>DSYVHRHVVTFDETNLVGNV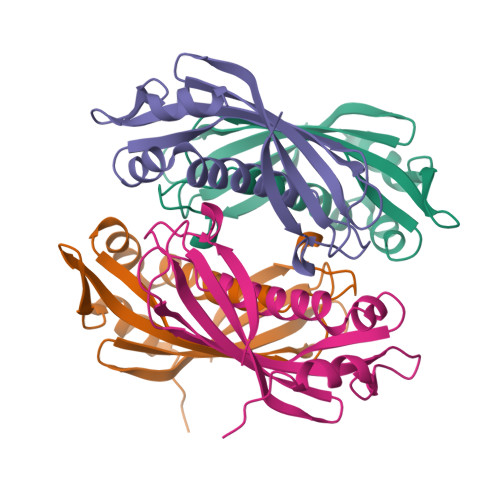YFAHYLHWQGHCREHFLADHAPGVMAALADGLALVTVDCHADFYAEGSAFDEVEVRMMLDRLDGHRIAMSFDYVRVAPGPPTLLAQGRQTVACMRRAGHGLEPVEVPAELRRALSRYAVVAR[8x]>[5x]GSSARQTAEQRQNLQAFRDY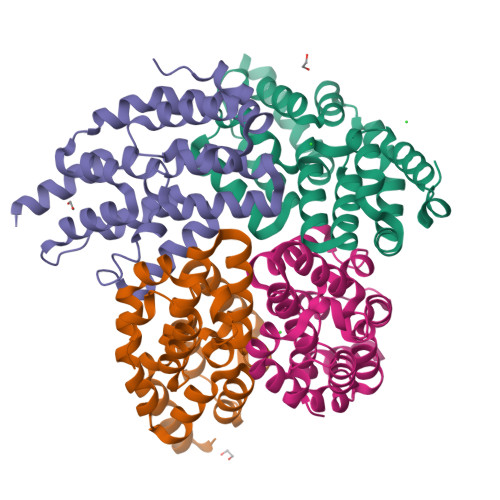IKKILDPTYILSYMSSWLEDEEVQYIQAEKNNKGPMEAASLFLQYLLKLQSEGWFQAFLDALYHAGYCGLCEAIESWDFQKIEKLEEHRLLLRRLEPEFKATVDPNDILSELSECLINQECEEIRQIRDTKGRMAGAEKMAECLIRSDKENWPKVLQLALEKDNSKFSELWIVD>[2x]GEFNTIQQLMMILNSASDQPSENLISYFNNCTVNPKESILKRVKDIGYIFKEKFAKAVGQGCVEIGSQRYKLGVRLYYRVMESMLKSEEERLSIQNFSKLLNDNIFHMSLLACALEVVMATYSRSTSQNLDSGTDLSFPWILNVLNLKAFDFYKVIESFIKAEGNLTREMIKHLERCKHRIMESLAWLSDSPLFDLIKQSKDREGPTDHLESACPLNLPLQNNHTAADMYLEPVRAPKKKSTSLSLFYKKVYRLAYLRLNTLCERLLSEHPELEHIIWTLFQHTLQNEYELMRDRHLDQIMMCSMYGICKVKNIDLKFKIIVTAYKDLPHAVQETFKRVLIKEEEYDSIIVFYNSVFMQRLKTNILQYASTRPPTLAPIPHIPRSPYKFP

The retinoblastoma tumor suppressor (Rb) is a multifunctional protein that primarily regulates the cell cycle but also has roles in cellular differentiation, DNA damage response, and apoptosis. Essential functions of Rb occur through its pocket domain, which is necessary for regulating binding interactions with E2F transcription factors and transcription repressors that bind via an LxCxE motif. The pocket domain is the most highly conserved region of the multidomain protein, as well as the most frequent site of mutations. Protein X-ray crystallography of four missense variants reveals how mutations destabilize the protein fold and inhibit E2FTD or LxCxE binding.

For E554K and E533K, we sought to understand the structural basis for large reductions in RbP-E2F1TD binding as well as substantial decreases in thermostability. The significance of E554 in Rb-E2FTD binding was initially pointed out by the authors of the two RbP-E2FTD structures as forming an H-bond the phenolic hydroxyl of conserved tyrosine in E2F1TD and E2F2TD. The structure of the cancer-associated variant, E554K, reveals how the lysine substitution disrupts the potential for these interactions by forming a shared salt bridge with E533 and E551. Remarkably, the crystal structure of E533K shows something similar in which the mutated lysine sidechain creates a salt bridge triad with E554 and E551 in a manner that occludes the Y411(E2F1TD)-binding pocket. Together, the variant structures of E533K and E554K reveal a structural basis for the disruption of E2FTD binding. However, from these structures alone, it is not clear how the mutations induce fold destabilization. In the structures of RbP-E2F2TD RbP-E2F1TD, both E554 and E533 form A/B subdomain-spanning salt bridges to K653. It is possible that the loss of the salt bridge interactions contributes to the large destabilization effects observed for these variants. Within the cyclin fold of subdomain A, the greatest destabilizing effects (ΔTm) are caused by E554K (−7.0 ± 0.5 °C), E533K (−6.4 ± 0.5 °C), E492Q (−5.4 ± 0.8 °C), A490V (−5.1 ± 0.6 °C), K462E (−5.0 ± 0.5 °C), E539D (−4.9 ± 0.5 °C), A490T (−4.7 ± 1.0 °C), and A488V (−4.1 ± 0.6 °C).>MSGFKFLFF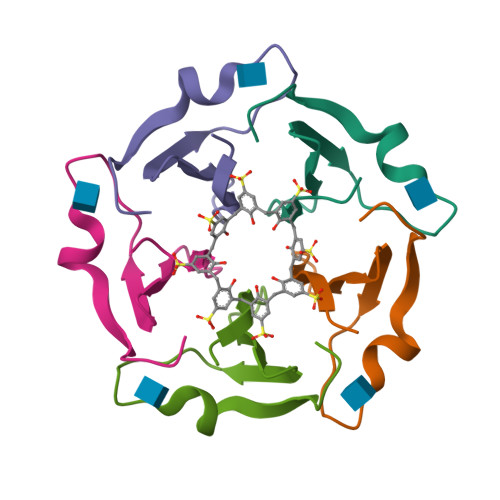SPDGTLYGVHNDKLYKGTPPTSDKDNWLARATLIGNGGW[10x]> MTKVVEISPTTRLEGHSKLTLKVNDQGIVERGDWLSITPVRGIEKLAIGKTMEQVPKIASRVCGICPIAHTLASTEAMEASIGCEIPTDAKLLRIILHAANRIHSHALHNILILPDFYIPGTEKKFNLFANEQPARSVMARIVRIREIAQTIAAIAGGEAIHPSNPRIGGMYHNVSPRAKQKMADLAKECLVLVHEQMEFMLDVIRNMQN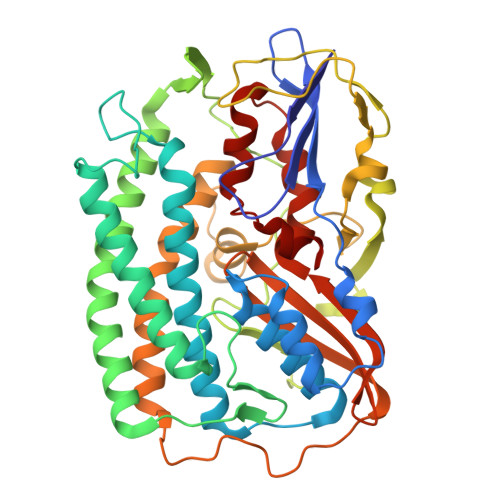REFVEVGGKQIPLPKKLGYHNQGVMATAPMYGSSSLDDNPTWDFTRWKETRPWDWYMGEVTIDLEDPSYPIGGTTKVGTKANPQMESCTGVPTYDGQPVEVGPRARLATFKNFDEKGTFAQHIARQMEYPDCCYTILNCLDNLNTSGKVLADHIPQGDGSMGWAANEAPRGSNIHLARVKDGKVRWYDMLVPTTWNFPTCSRALTGAPWQIAEMVVRAYDPCVSCATH>MASLAAEPSDVFIGLKIDQITGINQKEENFSVVGSLRIDWRQPLLAFEHAPGEPKHRTYTLATFLKLLEEKQIRWPAFTYHNQQGRMDFQNRLISLSEDGTVMYLERFTSTFQAPAFDFRLFPFDNQLFFIHVDSIFPQHLFRFQEMQGFSGLGDQLGEEEWIVTEVNTHLTTHNEFTKGDASRFVLEFHAERHLNYYLMRILIPVLLIITVSWFTFFLQDYTKRIDLAGGNLLLFIAFNFTISSDLPRLGYITLMDAFLVGTFIITALVV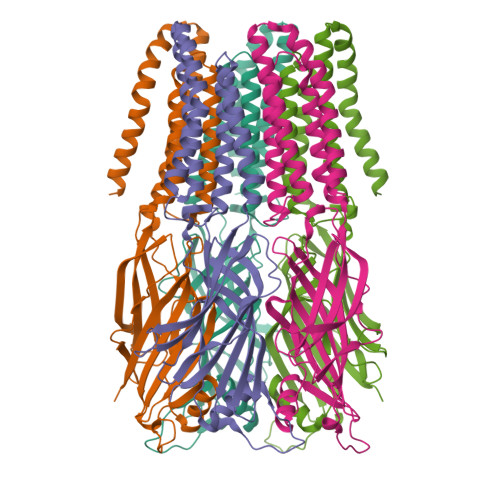LGNVWLRRLENHGKQALARKLDIYAITSYPLAYLLGALTLWLLFFWRSY[5x]> MTVFRQENVDDYYDTGEELGSGQFAVVKKCREKSTGLQYAAKFIKKRRTKSSRRGVSREDIEREVSILKEIQHPNVITLHEVYENKTDVILILELVAGGELFDFLAEKESLTEEEATEFLKQILNGVYYLHSLQIAHFDLKPENIMLLDRNVPKPRIKIIDFGLAHKIDFGNEFKNIFGTPEFVAPEIVNYEPLGLEADMWSIGVITYILLSGASPFLGDTKQE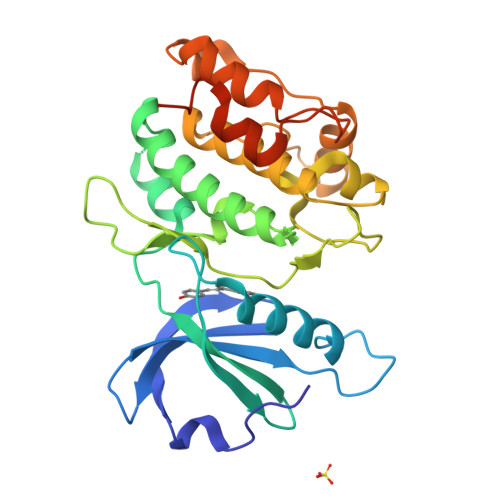TLANVSAVNYEFEDEYFSNTSALAKDFIRRLLVKDPKKRMTIQDSLQHPWIKPKDTQQALSLEHHHHHH> MNKVVLLCRPGFEKECAAEITDKAGQREIFGFARVKENAGYVIYECYQPDDGDKLIRELPFSSLIFARQWFVVGELLQHLPPEDRITPIVGMLQGVVEKGGELRVEVADTNESKELLKFCRKFTVPLRAALRDAGVLANYETPKRPVVHVFFIAPGCCYTGYSYSNNNSPFYMGIPRLKFPADAPSRSTLKLEE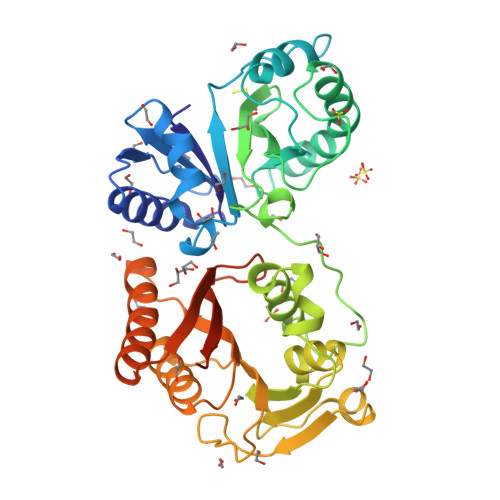AFHVFIPADEWDERLANGMWAVDLGACPGGWTYQLVKRNMWVYSVDNGPMAQSLMDTGQVTWLREDGFKFRPTRSNISWMVCDMVEKPAKVAALMAQWLVNGWCRETIFNLKLPMKKRYEEVSHNLAYIQAQLDEHGINAQIQARQLYHDREEVTVHVRRIWAAVGGRRDERSKGHHHHHH> LQPQEISPPPTANLDRSNDKVYENVTGLVKAVIEMSSKIQPAPPEEYVPMVKEVGLALRTLLATVDETI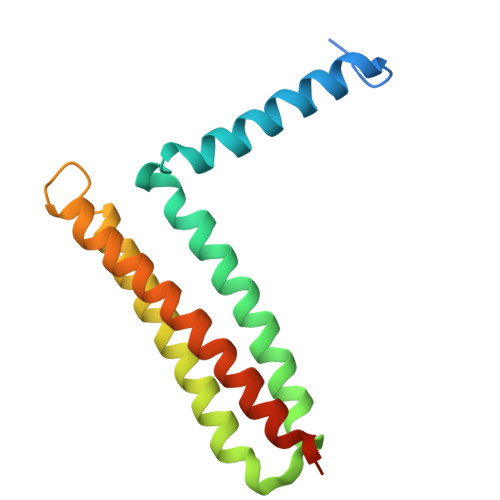PALPASTHREIEMAQKLLNSDLGELISKMKLAQQYVMTSLQQEYKKQMLTAAHALAVDAKNLLDVIDQARLKMLGQTRPH>[12x]MERFLLNSTVLLYRLSTVSLDEVSLDERVESSVFLAQYEQARSLPDHVAKSAWSYLVQQIKQRNMKLGPVAILRLIAEKFIKNEKGGPKIDLPMFSEWQTLMSRVSCLPIIACHQVFNPGPASQEYSFRWPLYPYHPTVEDYITRECLHETHQHLNGSTSAEECWLDALKHPEACLRDFEKGWASQEMKQLCAQIDPSLTPRIFKDRLQIACNIREILCRVAQGVELPEWIASMQNPQQLANSTILHNGREYGFATVWPIDDKYSQESEFCWLTGLLEKWRFNAPEGLERLLWIYLLIQNQYLTLLVQRDDFFGFEQFQNYTMTELREETEKSYLSRFKHAHGAGVYSQVRYLEGRFAPKSDPNKMQKLLFSVLRGYWEYLSAHMSMEWVHEKPLTISQVLDNLELVEPHGKCVELALVPHFIKRKPKNGEAYPHALLFKDLKNQAAILMDMLKSEPRLTGWIRGVDAAANEMHAPPELFCPLFRVLAKSGIAHFTYHVGEDFPHLISGIRSIDDALRFLPLRNGDRLGHCTAIGITPSIWKRSLPLSLSMTKETRLLDLVFIWRELRSHPELLRYASDAAIEAVRLAHKVFSLEEEVSITTLDQVFEMRGLLAESEGLLSELNEPLKPKSLWLEEYERARELVKTTGMKRPLKLYKQWLTSDNVRKQRAEYVEVALEYLPDEAVVALQQAVMAKMADRNIAIECPPTSNTRISQYRNVSEHHIFRWMGLPGEAIEGDVPMSICLGSDDPGIFAADLKSEFYHLFVVLTRKFGLSPADALRKVAEVNENGRIYRFHDV

The RADAR system comprises two genes, rdrA that encodes a protein with an ATPase domain, and rdrB, encoding a predicted adenosine deaminase domain protein. Here, we determine cryo-EM structures of the RADAR defense complex, revealing RdrA as a heptameric, two-layered AAA+ ATPase and RdrB as a dodecameric, hollow complex with twelve surface-exposed deaminase active sites. RdrA and RdrB join to form a giant assembly up to 10 MDa, with RdrA docked as a funnel over the RdrB active site. Our results define ATP mononucleotide deamination as a determinant of RADAR immunity and reveal supramolecular assembly of a nucleotide-modifying machine as a mechanism of anti-phage defense.

Cryo-EM analysis of E. coli RdrB showed an assembly of a rigid, higher-order complex, and we determined a structure to 2.1 Å. Structural analysis of the E. coli RdrB complex reveals three large insertions to the adenosine deaminase core that mediate higher order dodecameric assembly. Compared with a typical adenosine deaminase domain like Plasmodium vivax ADA (RMSD 2.4 Å),23 RdrB contains an N-terminal extension “insertion 1,” a unique “insertion 2” that divides the catalytic core, and an “insertion 3” after the final catalytic histidine H530. Insertions 1 and 2 form a 2-fold symmetrical interface that joins adjacent adenosine deaminase core domains. Insertion 3 forms a hydrophilic interface consisting of alternating glutamate and arginine residues that create a 3-fold symmetry axis and enable assembly of the large dodecameric shell. Some adenosine deaminases are known to function as dimers,24 but to the best of our knowledge, assembly of a large, shelled complex is a feature unique to RADAR RdrB. We made several mutations along the interfaces between RdrB protomers; charge disrupting mutations to the conserved glutamate residues that line interface 3 (E595R, E596R, and E597R) result in complete loss of anti-phage defense and demonstrate that RdrB complex assembly is essential for RADAR function. Comparison of E. coli RdrB against all structures in the Protein Data Bank (PDB) revealed that E. coli RdrB has no structural similarity to adenosine deaminases acting on RNA (ADAR) proteins, which are part of the cytidine deaminase superfamily of enzymes that use a mechanistically distinct active site to edit RNA. Instead, all the top hits with structural similarity to E. coli RdrB (Z score > 20) are adenosine or AMP deaminases that deaminate the adenosine within unphosphorylated or monophosphorylated monomeric substrates, as opposed to within RNA. HPLC analysis demonstrates that purified E. coli RdrB is alone sufficient to catalyze rapid conversion of ATP to ITP.> MMTFADKVIQFNKDLSYTGSTLPPGIRIMNPFKEHEQTMHIVEAFYHKYYNDNQSRYLILGINPGRFGSGLTGIPFTDPK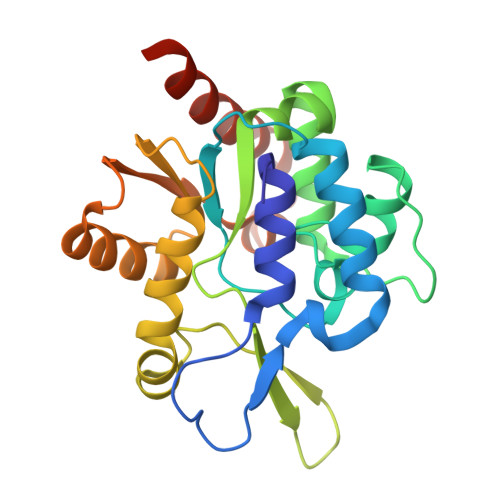RLITECNIPYSGKLSHEPSSVFIYEMINAFGGAEAFYKQFYISSPCPLGFTSIAANGKEKNYNYYDSKALEKAVYEFIIENIRKQLTLGITTDTCFCLGTGKNEKFLMKVNAQYKFFKRIVALEHPRFIMQYKTASKQFYIDKYISAFKALNNSAILEHHHHHH L-arabinitol | C5 H12 O5 | 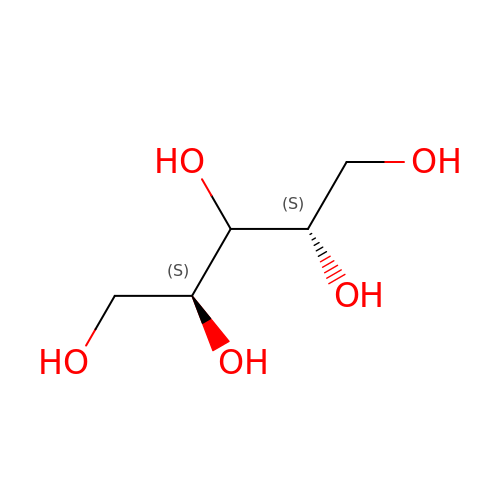HEBKCHPVOIAQTA-IMJSIDKUSA-N>KEEEDVICDGCNGPVVGTRYKCSVCPDYDLCSVCEGKGLHRGHTKLAFPSPFGHLSEGFS[2x]

Intriguingly, the autophagy adapter p62/SQSTM1/Sequestosome-1 was recently reported to recognize N-degrons, the N-end rule substrates of the well-characterized UPS, and where ultimately these substrates are delivered to ALS8,9. p62 is a key selective autophagy adapter that plays a role in the degradation of various cellular constituents such as misfolded proteins and their aggregates, malfunctioning organelles, and invading pathogens. Intriguingly, it was recently reported that the central ZZ-domain in p62 plays a critical role in the recognition of N-terminal arginylated BiP/GRP78 by the Arg-tRNA transferase ATE1. Here, we present the high resolution structures of the ZZ-domain of p62 in complex with 8 different N-degrons including type-1 and type-2, and subsequently identify key determinants involved in the unusual recognition.

Therefore, we determined the structure of the ZZ-domain in complex with a variety of N-degrons comprising three type-1 N-degrons and five type-2 N-degrons. As described for the R-BiP complex, two aspartic acid residues, Asp129 and Asp149, bind to the α-amino group, and Asp147 forms a hydrogen bond with the first peptide bond, which means that these interactions are conserved in all different N-terminal residues. However, the side chain of the N-terminal residue of the N-degron is recognized differently. The side chain of Asn132 which undergoes a conformational change plays a critical role in interacting with the first residue of the N-degron. The bipolar nature of the side chain atoms (O and N) of Asn132 allow for the recognition of positively charged type-1 substrates as well as type-2 substrates, and especially N-terminal tyrosine and tryptophan residues since they possess polar atoms in the side chain. The binding affinity between the ZZ-domain and other type-1 substrates with histidine or lysine residues at the primary position showed ca. a 10-fold reduction, although it was still significant.>SLTQEQLEDARRLKAIWEKKKNELGLSYESVADKMGMGQSAVAALFNGINALNAYNAALLAKILKVSVEEFSPSIAREIR[2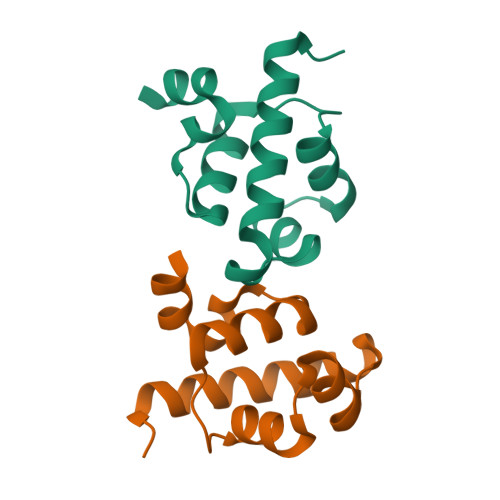x]TAZOBACTAM TRANS-ENAMINE INTERMEDIATE | C10 H14 N4 O5 S | 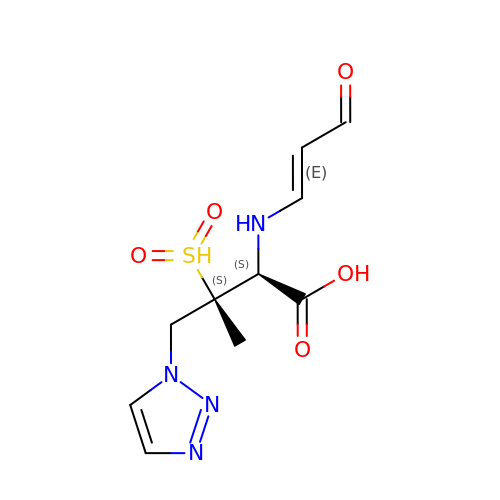ANZZKUOZZHRUQC-QZWDGIGVSA-N> GQ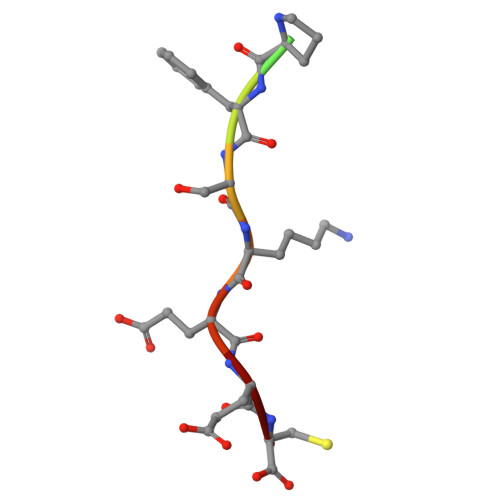VPFSKEEC Bacteriophage exclusion (‘BREX’) systems are multi-protein complexes encoded by a variety of bacteria and archaea that restrict phage by an unknown mechanism. The final gene in most type 1 BREX systems, termed ‘BrxL’, encodes a large protein (670–700 residues in various species), with much of its sequence predicted to adopt a fold corresponding to the chambered ATP-dependent AAA+ protein family, which are involved in a wide variety of cellular functions throughout all biological kingdoms. In this study we have demonstrated that the BrxL phage restriction factor is a multimeric DNA binding protein that displays ATP-dependent assembly on double stranded DNA.

To better understand how BrxL’s C-terminal domain relates to those or other protein domains (and to provide a starting model of that domain for subsequent CryoEM studies of the full-length protein) we expressed, purified, and crystallized BrxLC. During the final step of purification by size exclusion chromatography (SEC), we observed that BrxLC eluted at a retention volume consistent with a monomer rather than as a higher order multimers (eventually shown to correspond to hexamers) previously observed in studies of LonPC and RadAC. We obtained crystals and solved the X-ray structure to 2.25 Å resolution. The crystal structure contains 4 subunits in the asymmetric unit, with no obvious higher order symmetry. The backbone atoms of BrxLC superpose well with both domains despite low amino acid sequence identity (BrxLC shares 14% identity with both domains); superposition of BrxLC with RadC generates an RMSD value for 148 structurally equivalent α-carbons of 2.3 Å (P-value 8.97 × 10−14); superposition with LonPC generates an RMSD value for 172 structurally equivalent α-carbons of 3.3 Å (P-value 3.02 × 10−12). A structure-based sequence alignment of the BrxLC with RadAC or LonPC does not demonstrate obvious conservation with previously visualized DNA binding residues with RadAC or with a protease catalytic motif as observed in LonPC. BrxLC’s distinct solution and assembly behaviors, in conjunction with the low sequence conservation relative to LonPC and RadAC, indicate that the BrxLC domain may have adopted a distinct structural role in the function of BrxL as compared to the same domain in LonP or RadA. In contrast, purified BrxLC is monomeric in solution and (in the context of full-length BrxL) appears to mediate dimerization of heptameric (without ATP) or hexameric (with ATP) complexes through protein-protein interactions with another BrxLC partner. In the DNA-bound dodecameric complex, BrxLc domains are far removed from dsDNA occupying the central pore and do not share significant conservation with LonP residues essential for protease activity or with RadA residues involved in DNA binding. These observations imply that BrxL’s CTD has evolved a distinct functional role from the LonPC and RadAC domains.

>GSHMKPGFLYTIGLSNKGMPGLYRLELQVTKGSGKLATSGLWNSSSAKEQVKIAFDYFKANASRISGGSKVMEHDFHLHVVELQNTGPLSHLALPSLVAFASGLLGRSVQSQMVVLGDMSLGGSVTPVESIAECLQVAFDAGAKKVALPMSSAADIPTIPVELFTKFQTSFYADPVDAVFKGLGVD[4x]>[22x]MSSLLNSLLPEYFKPKTNLNINSSRVQYGFNARIDMQYEDDSGTRKGSRPNAFMSNTVAFIGNYEGIIVDDIPILDGLRADIFDTHGDLDMGLVEDALSKST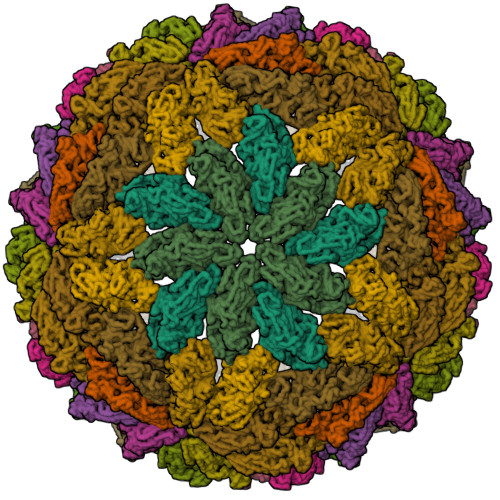MIRRNVPTYTAYASELLYKRNLTSLFYNMLRLYYIKKWGSIKYEKDAIFYDNGHACLLNRQLFPKSRDASLESSLSLPEAEIAMLDPGLEFPEEDVPAILWHGRVSSRATCILGQACSEFAPLAPFSIAHYSPQLTRKLFVNAPAGIEPSSGRYTHEDVKDAITILVSANQAYTDFEAAYLMLAQTLVSPVPRTAEASAWFINAGMVNMPTLSCANGYYPALTNVNPYHRLDTWKDTLNHWVAYPDMLFYHSVAMIESCYVELGNVARVSDSDAINKYTFTELSVQGRPVMNRGIIVDLTLVAMRTGREISLPYPVSCGLTRTDALLQGTEIHVPVVVKDIDMPQYYNAIDKDVIEGQETVIKVKQLPPAMYPIYTYGINTTEFYSDHFEDQVQVEMAPIDNGKAVFNDARKFSKFMSIMRMMGNDVTATDLVTGRKVSNWADNSSGRFLYTDVKYEGQTAFLVDMDTVKARDHCWVSIVDPNGTMNLSYKMTNFRAAMFSRNKPLYMTGGSVRTIATGNYRDAAERLRAMDETLRLKPFKITEKLDFRVAAYAIPSLSGSNMPSLHHQEQLQISEVDAEPINPIGEDELPPDIE> MSPVGRLFLGSKLPAQTWQSFRLQPALPQFAQKRFFSGGAAKPSWHVAREHRFGPTLPDHAYYGEHATYNYFVLFIRGMRP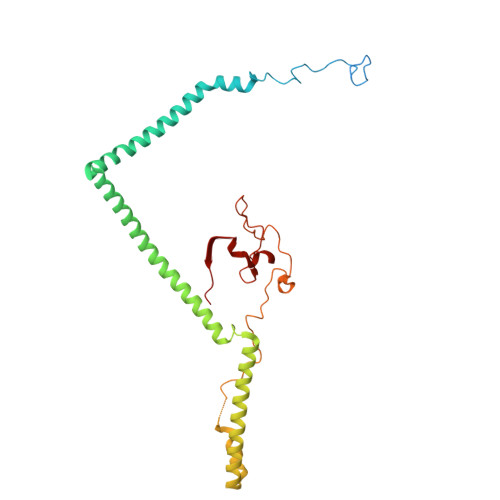YLEKIFGDCASTIKNAAVAVYRPVNAFVVKHNPDLRLQFVAFASFIATHMAITKEFNDMYQRLVDITSLLELQAAQLHASEGFWDSESEQQEARLQRHAEHRNDLETTWEEALREATLARNFDVLVSYLNHGTSDGCGEHGACGHSGQNGIPPSVTWNFNAMPYGKENPDTKTFPIPDHEQPYRAFSLGFTANNLSGNWGDYIDRQDNKNALMRPARMMFTDVFIPTTK>MKKIWLALAGLVLAFSASAAQYEDGKQYTTLEKPVAGAPQVLEFFSFFCPHCYQFEEVLHISDNVKKKLPEGVKMTKYHVNFMGGDLGKDLTQAWAVAMALGVEDKVTVPLFEGVQKTQTIRSASDIRDVFINAGIKGEEYDAAWNSFVVKSLVAQQEKAAADVQLRGVPAMFVNGKYQLNPQGMD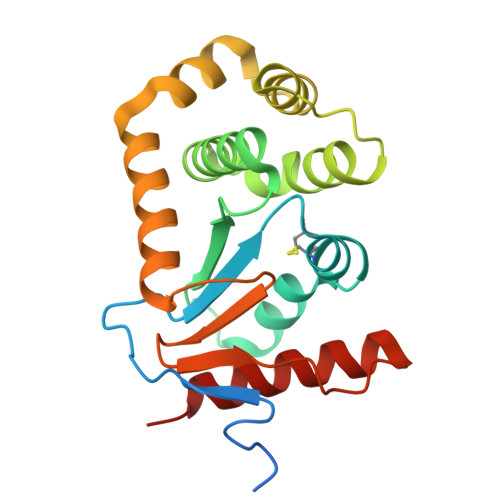TSNMDVFVQQYADTVKYLSEKK[2x]> SILWHEMWHEGLEEASRLYFGERNVK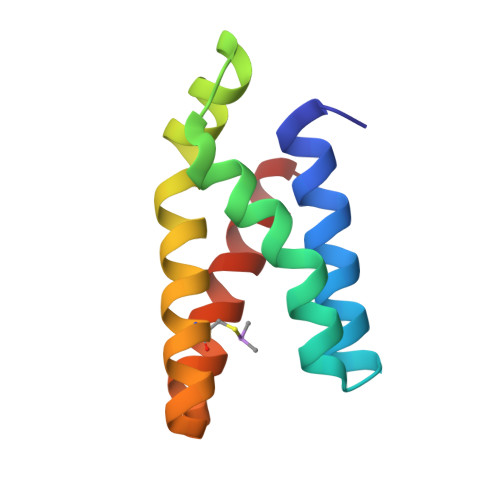GMFEVLEPLHAMMERGPQTLKETSFNQAYGRDLMEAQEWCRKYMKSGNVKDLTQAWDLYYHVFRRIS[[(2R,3S,4R,5R)-5-(6-aminopurin-9-yl)-3,4-dihydroxyoxolan-2-yl]methoxy-hydroxyphosphoryl] 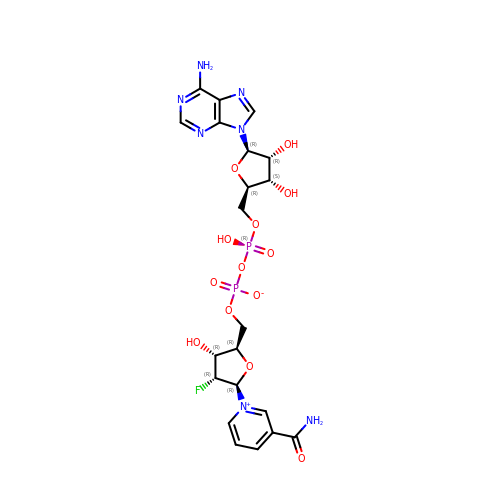[(2R,3S,4R,5R)-5-(3-carbamoylpyridin-1-ium-1yl)- 3-fluoro-,4- hydroxyoxolan-2-yl]methyl phosphate | C21 H26 F N7 O13 P2 | JSGNSBZQCQQLEF-OZCXFSBSSA-N>[6x]MERLRQIAS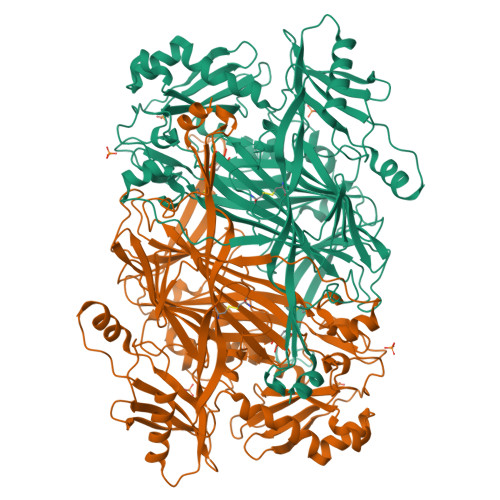QATAASAAPARPAHPLDPLSTAEIKAATNTVKSYFAGKKISFNTVTLREPARKAYIQWKEQGGPLPPRLAYYVILEAGKPGVKEGLVDLASLSVIETRALETVQPILTVEDLCSTEEVIRNDPAVIEQCVLSGIPANEMHKVYCDPWTIGYDERWGTGKRLQQALVYYRSDEDDSQYSHPLDFCPIVDTEEKKVIFIDIPNRRRKVSKHKHANFYPKHMIEKVGAMRPEAPPINVTQPEGVSFKMTGNVMEWSNFKFHIGFNYREGIVLSDVSYNDHGNVRPIFHRISLSEMIVPFGSPEFPHQRKHALDIGEYGAGYMTNPLSLGCDCKGVIHYLDAHFSDRAGDPITVKNAVCIHEEDDGLLFKHSDFRDNFATSLVTRATKLVVSQIFTAANXEYCLYWVFMQDGAIRLDIRLTGILNTYILGDDEEAGPWGTRVYPNVNAHNHQHLFSLRIDPRIDGDGNSAAACDAKSSPYPLGSPENMYGNAFYSEKTTFKTVKDSLTNYESATGRSWDIFNPNKVNPYSGKPPSYKLVSTQCPPLLAKEGSLVAKRAPWASHSVNVVPYKDNRLYPSGDHVPQWSGDGVRGMREWIGDGSENIDNTDILFFHTFGITHFPAPEDFPLXPAEPITLMLRPRHFFTENPGLDIQPSYAMTTSEAKRAVHKETKDKTSRLAFEGSCCGK> GGGSMEPGRGGTETVGKFEFSRKDLIGHGAFAVVFKGRHRAAHDLEVAVKCINKKNLAKSQTLLGKEIKILKELKHENIVALYDFQEMANSVYLVMEYCNGGDLADYLHAMRTLSEDTIRLFLQQIAGAMRLLHSKGIIHRDLKPQNILLSNPAGRRANPNSIRVKIADFGFARYLQSNMMAATLCG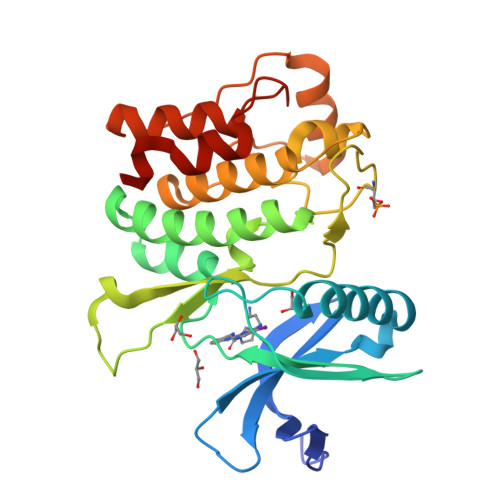SPMYMAPEVIMSQHYDGKADLWSIGTIVYQCLTGKAPFQASSPQDLRLFYEKNKTLVPTIPRETSAPLRQLLLALLQRNHKDRMDFDEFFHHPFLDASPS> AKWVCKICGYIYDEDAGDPDNGIS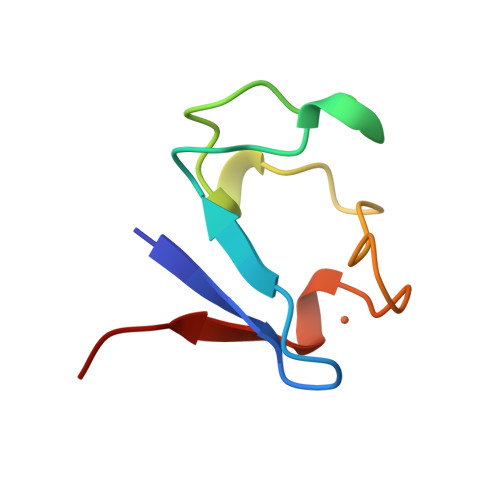PGTKFEELPDDWVCPICGAPKSEFEKLED> IVGGQECKDGECPWQALLINEENEGFCGGTILSEFYILTAAHCLYQAKRFKVRVGDRNTEQEEGGEAVHEVEVVIKHNRFTKETYDFDIAVLRLKTPITFRMNVAPACLPERDWAESTLMTQKTG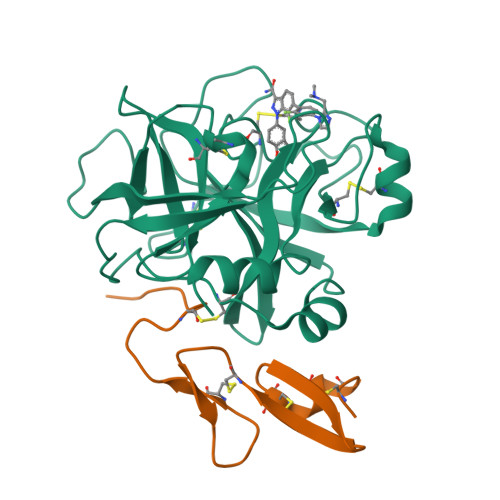IVSGFGRTHEKGRQSTRLKMLEVPYVDRNSCKLSSSFIITQNMFCAGYDTKQEDACQGDSGGPHVTRFKDTYFVTGIVSWGEGCARKGKYGIYTKVTAFLKWIDRSMKT;> VCSLDNGDCDQFCHEEQNSVVCSCARGYTLADNGKACIPTGPYPCGKQTLE>MSEKTTKGVQLLRGDPKKAIVRLSIPMMIGMSVQTLYNLADGIWVSGLGPESLAAVGLFFPVFMGIIALAAGLGVGTSSAIARRIGARDKEGADNVAVHSLILSLILGVTITITMLPAIDSLFRSMGAKGEAVELAIEYARVLLAGAFIIVFNNVGNGILRGEGDANRAMLAMVLGSGLNIVLDPIFIYTLGFGVVGAAYATLLSMVVTSLFIAYWLFVKRDTYVDITLRDFSPSREILKDILRVGLPSSLSQLSMSIAMFFLNSVAITAGGENGVAVFTSAWRITMLGIVPILGMATATTSVTGAAYGERNVEKLETAYLYAIKIAFMIELAVVAF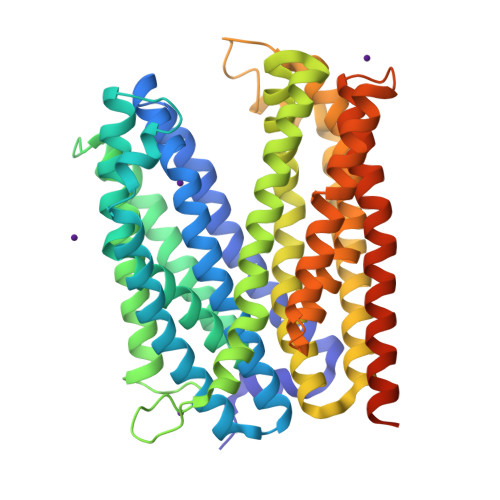IMLFAPQVAYLFTYSESAQVIKGDLISALRTLPVFLVLTPFGMMTSAMFQGIGEGEKSLILTIFRTLVMQVGFAYIFVHYTTLGLRGVWIGIVIGNMVAAIVGFLWGRMRISALKKTSATGGKRRNSENLYFQGGRGSHHHHHHHHHH[4x]>MDQKQFEKIRAVFDRSGVALTLVDMSLPEQPLVLANPPFLRMTGYTEGQILGFNCRFLQRGDENAQARADIRDALKLGRELQVVLRNYRANDEPFDNLLFLHPVGGRPDAPDYFLGSQFELGRSGNSEEAAAAGHAGYLTGELARIGTVAARLEMDSRRHLAQAAAALVRAWER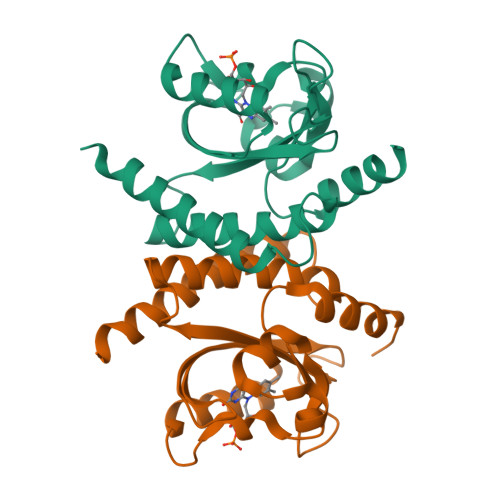RG[2x]>MRGIILAGGSGTRLYPITMGISKQLLPVYDKPMIYYPLTTLMMAGIRDIQLITTPHDAP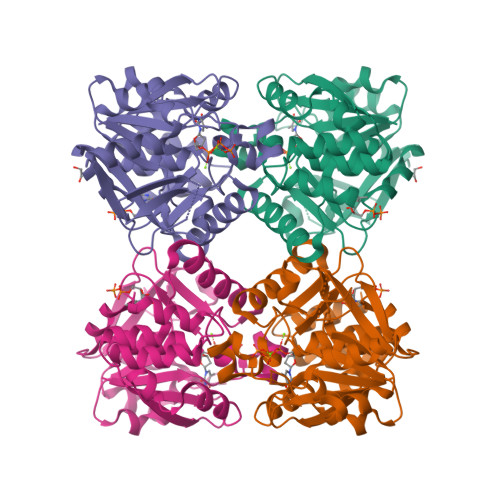GFHRLLGDGAHLGVNISYATQDQPDGLAQAFVIGANHIGADSVALVLGDNIFYGPGLGTSLKRFQSISGGAIFAYWVANPSAYGVVEFGAEGMALSLEEKPVTPKSNYAVPGLYFYDNDVIEIARGLKKSARGEYEITEVNQVYLNQGRLAVEVLARGTAWLDTGTFDSLLDAADFVRTLERRQGLKVSIPEEVAWRMGWIDDEQLVQRARALVKSGYGNYLLELLERNLEHHHHHH[2x]pinocembrin 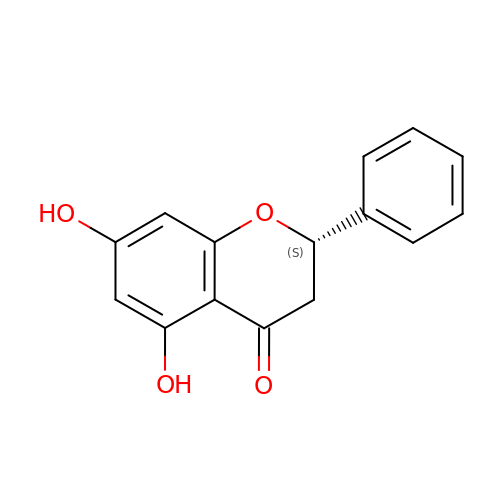| C15 H12 O4 | URFCJEUYXNAHFI-ZDUSSCGKSA-N>[2x]MQEILIPLKEKNYKVFLGELPEIKLKQKALIISDSIVAGLHLPYLLERLKALEVRVCVIESGEKYKNFHSLERILNNAFEMQLNRHSLMIALGGGVISDMVGFASSIYFRGIDFINIPTTLLAQVDASVGGKTGINTPYGKNLIGSFHQPKAVYMDLAFLKTLEKREFQAGVAEIIKMAVCFDKNLVERLETKDLKDCLEEVIFQSVNIKAQVVVQDEKEQNIRAGLNYGHTFGHAI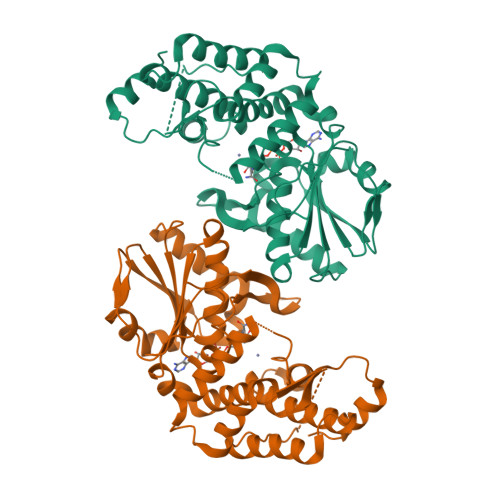EKETDYERFLHGEAIAIGMRMANDLALSLGMLTLKEYERIENLLKKFDLIFHYKILDLQKFYERLFLDKKSENKTIKFILPKGVGAFEVASHIPKETIIKVLEKWH6-(2,6-DICHLOROPHENYL)-2-[(4-FLUORO-3-METHYLPHENYL)AMINO]-8-METHYLPYRIDO[2,3-D]PYRIMIDIN-7(8H)-ONE | C21 H15 Cl2 F N4 O | 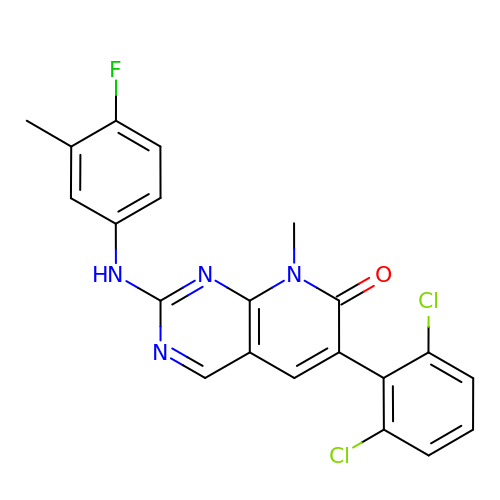SLCFEJAMCRLYRG-UHFFFAOYSA-N> MMETERLVLPPPDPLDLPLRAVELGCTGHWELLNLPGAPESSLPHGLPPCAPDLQQEAEQLFLSSPAWLPLHGVEHSARKWQRKTDPWSLLAVLGAPVPSDLQAQRHPTTGQILGYKEVLLENTNLSATTSLSLRRPPGPASQSLWGNPTQYPFWPGGMDEPTITDLNTREEAEEEIDFEKDLLTIPPGFKKGMDFAPKDCPTPAPGLLSLSCMLEPLDLGGGDEDENEAVGQPGGPRGDTVSASPCSAPLARASSLEDLVLKEASTAVSTP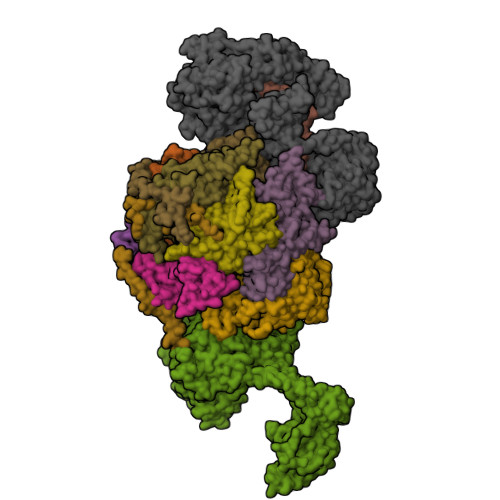EAPEPPSQEQWAIPVDATSPVGDFYRLIPQPAFQWAFEPDVFQKQAILHLERHDSVFVAAHTSAGKTVVAEYAIALAQKHMTRTIYTSPIKALSNQKFRDFRNTFGDVGLLTGDVQLHPEASCLIMTTEILRSMLYSGSDVIRDLEWVIFDEVHYINDVERGVVWEEVLIMLPDHVSIILLSATVPNALEFADWIGRLKRRQIYVISTVTRPVPLEHYLFTGNSSKTQGELFLLLDSRGAFHTKGYYAAVEAKKERMSKHAQTFGAKQPTHQGGPAQDRGVYLSLLASLRTRAQLPVVVFTFSRGRCDEQASGLTSLDLTTSSEKSEIHLFLQRCLARLRGSDRQLPQVLHMSELLNRGLGVHHSGILPILKEIVEMLFSRGLVKVLFATETFAMGVNMPARTVVFDSMRKHDGSTFRDLLPGEYVQMAGRAGRRGLDPTGTVILLCKGRVPEMADLHRMMMGKPSQLQSQFRLTYTMILNLLRVDALRVEDMMKRSFSEFPSRKDSKAHEQALAELTKRLGALEEPDMTGQLVDLPEYYSWGEELTETQHMIQRRIMESVNGLKSLSAGRVVVVKNQEHHNALGVILQVSSNSTSRVFTTLVLCDKPLSQDPQDRGPATAEVPYPDDLVGFKLFLPEGPCDHTVVKLQPGDMAAITTKVLRVNGEKILEDFSKRQQPKFKKDPPLAAVTTAVQELLRLAQAHPAGPPTLDPVNDLQLKDMSVVEGGLRARKLEELIQGAQCVHSPRFPAQYLKLRERMQIQKEMERLRFLLSDQSLLLLPEYHQRVEVLRTLGYVDEAGTVKLAGRVACAMSSHELLLTELMFDNALSTLRPEEIAALLSGLVCQSPGDAGDQLPNTLKQGIERVRAVAKRIGEVQVACGLNQTVEEFVGELNFGLVEVVYEWARGMPFSELAGLSGTPEGLVVRCIQRLAEMCRSLRGAARLVGEPVLGAKMETAATLLRRDIVFAASLYTQ;> GPDSSQCESPSLTELFQEHKENNISQCFTLSDLCNQSSASFTDLSLGSFPLSQLANRCQSSPGISELTGSLSSLAFHKASPTRDLENLSLSELIAETIDVDNSQIKKESFEVSLSEVRSPGIDSNIDLSVLIKNPDFVPKPVVDPSIAPSSRTKVLSSKLGKNSNFAKDNKKNNKGSLTRKPPFSLSWTKALAARPSAFASTLCLRYPLKSCKRRTLDLYKTFLYSRQVQDVKDKEISPLVAITPFDFKSASPDDIVKANQKKAFTRELEVLFQ;> GPDSMASVTLSEAEKVYIVHGVQEDLRVDGRGCEDYRCVEVETDVVSNTSGSARVKLGHTDILVGVKAEMGTPKLEKPNEGYLEFFVDCSASATPEFEGRGGDDLGTEIANTLYRIFNNKSSVDLKTLCISPREHCWVLYVDVLLLECGGNLFDAISIAVKAALFNTRIPRVRVLEDEEGSKDIELSDDPYDCIRLSVENVPCIVTLCKIGYRHVVDATLQEEACSLASLLVSVTSKGVVTCMRKVGKGSLDPESIFEMMETGKRVGKVLHASLQSVVHKEESLGPKRQKVGFLG;> MPGDHRRIRGPEESQPPQLYAADEEEAPGTRDPTRLRPVYARAGLLSQAKGSAYLEAGGTKVLCAVSGPRQAEGGERGGGPAGAGGEAPAALRGRLLCDFRRAPFAGRRRRAPPGGCEERELALALQEALEPAVRLGRYPRAQLEVSALLLEDGGSALAAALTAAALALADAGVEMYDLVVGCGLSLAPGPAPTWLLDPTRLEEERAAAGLTVALMPVLNQVAGLLGSGEGGLTESWAEAVRLGLEGCQRLYPVLQQSLVRAARRRGAAAQP;> GPDSMAEPASVAAESLAGSRARAARTVLGQVVLPGEELLLPEQEDAEGPGGAVERPLSLNARACSRVRVVCGPGLRRCGDRLLVTKCGRLRHKEPGSGSGGGVYWVDSQQKRYVPVKGDHVIGIVTAKSGDIFKVDVGGSEPASLSYLSFEGATKRNRPNVQVGDLIYGQFVVANKDMEPEMVCIDSCGRANGMGVIGQDGLLFKVTLGLIRKLLAPDCEIIQEVGKLHPLEIVFGMNGRIWVKAKTIQQTLILANILEACEHMTSDQRKQIFSRLAES;> GPDSMAMEMRLPVARKPLSERLGRDTKKHLVVPGDTITTDTGFMRGHGTYMGEEKLIASVAGSVERVNKLICVKALKTRYIGEVGDIVVGRITEVQQKRWKVETNSRLDSVLLLSSMNLPGGELRRRSAEDELAMRGFLQEGDLISAEVQAVFSDGAVSLHTRSLKYGKLGQGVLVQVSPSLVKRQKTHFHDLPCGASVILGNNGFIWIYPTPEHKEEEAGGFIANLEPVSLADREVISRLRNCIISLVTQRMMLYDTSILYCYEASLPHQIKDILKPEIMEEIVMETRQRLLEQEG;> GPDSMAPPVRYCIPGERLCNLEEGSPGSGTYTRHGYIFSSLAGCLMKSSENGALPVVSVVRETESQLLPDVGAIVTCKVSSINSRFAKVHILYVGSMPLKNSFRGTIRKEDVRATEKDKVEIYKSFRPGDIVLAKVISLGDAQSNYLLTTAENELGVVVAHSESGIQMVPISWCEMQCPKTHTKEFRKVARVQPEFLQT;> GPDSMKETPLSNCERRFLLRAIEEKKRLDGRQTYDYRNIRISFGTDYGCCIVELGKTRVLGQVSCELVSPKLNRATEGILFFNLELSQMAAPAFEPGRQSDLLVKLNRLMERCLRNSKCIDTESLCVVAGEKVWQIRVDLHLLNHDGNIIDAASIAAIVALCHFRRPDVSVQGDEVTLYTPEERDPVPLSIHHMPICVSFAFFQQGTYLLVDPNEREERVMDGLLVIAMNKHREICTIQSSGGIMLLKDQVLRCSKIAGVKVAEITELILKALENDQKVRKEGGKFGFAESIANQRITAFKMEKAPIDTSDVEEKAEEIIAEAEPPSEVVSTPVLWTPGTAQIGEGVENSWGDLEDSEKEDDEGGGDQAIILDGIKMDTGVEVSDIGSQDAPIILSDSEEEEMIILEPDKNPKKIRTQTTSAKQEKAPSKKPVKRRKKKRAAN;> MAGLELLSDQGYRVDGRRAGELRKIQARMGVFAQADGSAYIEQGNTKALAVVYGPHEIRGSRARALPDRALVNCQYSSATFSTGERKRRPHGDRKSCEMGLQLRQTFEAAILTQLHPRSQIDIYVQVLQADGGTYAACVNAATLAVLDAGIPMRDFVCACSAGFVDGTALADLSHVEEAAGGPQLALALLPASGQIALLEMDARLHEDHLERVLEAAAQAARDVHTLLDRVVRQHVREASILLGD;> GPMLQKREKVLLLRTFQGRTLRIVREHYLRPCVPCHSPLCPQPAACSHDGKLLSSDVTHYVIPDWKVVQDYLEILEFPELKGIIFMQTACQAVQHQRGRRQYNKLRNLLKDARHDCILFANEFQQCCYLPRERGESMEKWQTRSIYNAAVWYYHHCQDRMPIVMVTEDEEAIQQYGSETEGVFVITFKNYLDNFWPDLKAAHELCDSILQSRRERENESQESHGKEYPEHLPLEVLEAGIKSGRYIQGILNVNKHRAQIEAFVRLQGASSKDSDLVSDILIHGMKARNRSIHGDVVVVELLPKNEWKGRTVALCENDCDDKASGESPSEPMPTGRVVGILQKNWRDYVVTFPSKEEVQSQGKNAQKILVTPWDYRIPKIRISTQQAETLQDFRVVVRIDSWESTSVYPNGHFVRVLGRIGDLEGEIATILVENSISVIPFSEAQMCEMPVNTPESPWKVSPEEEQKRKDLRKSHLVFSIDPKGCEDVNDTLSVRTLNNGNLELGVHIADVTHFVAPNSYIDIEARTRATTYYLADRRYDMLPSVLSADLCSLLGGVDRYAVSIMWELDKASYEIKKVWYGRTIIRSAYKLFYEAAQELLDGNLSVVDDIPEFKDLDEKSRQAKLEELVWAIGKLTDIARHVRAKRDGCGALELEGVEVCVQLDDKKNIHDLIPKQPLEVHETVAECMILANHWVAKKIWESFPHQALLRQHPPPHQEFFSELRECAKAKGFFIDTRSNKTLADSLDNANDPHDPIVNRLLRSMATQAMSNALYFSTGSCAEEEFHHYGLALDKYTHFTSPIRRYSDIVVHRLLMAAISKDKKMEIKGNLFSNKDLEELCRHINNRNQAAQHSQKQSTELFQCMYFKDKDPATEERCISDGVIYSIRTNGVLLFIPRFGIKGAAYLKNKDGLVISCGPDSCSEWKPGSLQRFQNKITSTTTDGESVTFHLFDHVTVRISIQASRCHSDTIRLEIISNKPYKIPNTELIHQSSPLLKSELVKEVTKSVEEAQLAQEVKVNIIQEEYQEYRQTKGRSLYTLLEEIRDLALLDVSNNYGI;> GPDSMAAGFKTVEPLEYYRRFLKENCRPDGRELGEFRTTTVNIGSISTADGSALVKLGNTTVICGVKAEFAAPSTDAPDKGYVVPNVDLPPLCSSRFRSGPPGEEAQVASQFIADVIENSQIIQKEDLCISPGKLVWVLYCDLICLDYDGNILDACTFALLAALKNVQLPEVTINEETALAEVNLKKKSYLNIRTHPVATSFAVFDDTLLIVDPTGEEEHLATGTLTIVMDEEGKLCCLHKPGGSGLTGAKLQDCMSRAVTRHKEVKKLMDEVIKSMKPK;> GPDSMEEETHTDAKIRAENGTGSSPRGPGCSLRHFACEQNLLSRPDGSASFLQGDTSVLAGVYGPAEVKVSKEIFNKATLEVILRPKIGLPGVAEKSRERLIRNTCEAVVLGTLHPRTSITVVLQVVSDAGSLLACCLNAACMALVDAGVPMRALFCGVACALDSDGTLVLDPTSKQEKEARAVLTFALDSVERKLLMSSTKGLYSDTELQQCLAAAQAASQHVFRFYRESLQRRYSKS>TSEFPYKVDAKYQRYNSLKNFFEKTFDPEANKTPIKFHYDDVSKITGKKDTGKDLPTLNAERLGIKGRPATHTETSILFHTQHLGAMLTQRHNETGWTGLDEALNAGAWAVEFDYSGFNATGGGPGSVIPLYPINPMTNEIANEPVMVPGLYNWDNIDVESVRQQGQQWKFESKEEASKIVKKATRLLGADLVGIAPYDERWTYSTWGRKIYKPCKMPNGRTKYLPWDLPKMLSGGGVEVFGHAKFEPDWEKYAGFKPKSVIVFVLEEDYEAIRTSPSVISSATVGKSYSNMAEVAYKIAVFLRKLGYYAAPCGNDTGISVPMAVQAGLGEAGRNGLLITQKFGPRHRIAKVYTDLELAPDKPRKFGVREFCRLCKKCADACPAQAISHEKDPKVLQPEDCEVAENPYTEKWHLDSNRCGSFWAYNGSPCSNCVAVCSWNKVETWNHDVARIATQIPLLQDAARKFDEWFGYNGPVNPDERLESGYVQNMVKDFWNNPESIKQ[2x];>MNIYDVLIWMALGMTALLIQYGIWRYLKGKGKDTIPLQICGFLANFFFIFALAWGYSSFSEREYQAIGMGFIFFGGTALIPAIITYRLA[2x]

The major players in this process are respiratory reductive dehalogenases, corrinoid enzymes that use organohalides as substrates and contribute to energy conservation. The key enzyme in this dissimilatory pathway is the reductive dehalogenase (RDase), a membrane-associated protein that is facing the P-side of the cytoplasmic membrane after transport via the Twin-arginine translocation (Tat) system. The active site of RDases has a cobalt corrinoid cofactor that mediates halogen elimination or substitution, and two additional iron-sulphur (FeS) clusters for intramolecular electron transfer. Here, we show the structure of a menaquinol:organohalide oxidoreductase (MOOR) complex isolated from D. hafniense strain TCE1 as a dimer of heterodimers (PceA2B2).

A subset of the data containing 34’078 particles was retrieved, from which the 3D refinement produced a C2 map with an overall resolution of 2.83 Å. The large PceA subunit has a globular shape structured with α- and β-folds, while PceB has three TMH predicted to be fully integrated into the lipid bilayer, thus acting as the membrane anchor for the complex. Unexpectedly, electron density for two menaquinone molecules was also observed, each at the interface between PceA and PceB subunits. Finally, density for a dichloroethene (DCE) molecule, the final product of PCE dechlorination, was observed 5.3 Å away from each of the two active site cobalt atoms. In our structure, the catalytic site is 8.3 Å apart from the proximal FeS cluster, that is 9.9 Å away from the distal FeS cluster, which in turn is aligned with the menaquinol hydroxyl groups with distances shorter than 12 Å. This organisation forms a conductive redox path between the menaquinol pool and the active site. In the PceA C-terminal domain (S486-Q551), two α-helices predicted to be embedded in the membrane (α17 and α18) lay close to each other at a 53° angle, and bind a menaquinone molecule between them. Interestingly, in the quinone-binding site, three polar amino acids seem to stabilise the quinone head, due to their proximity to the molecule polar groups: K489 (at 3.7 Å), H495 (2.5 Å), R499 (5.4 Å) and D515 (4.5 Å). In contrast, we think that these residues, together with conserved residues in PceA (H495, D515, Y520), could be involved in the transfer of protons from the MKH2 oxidation to the P-side of the membrane.>GAIRSDFSNEDIYDNIDPDTISFPPKIATTDLFLPLFFHFGSTRQFMDKLHEVISGDYEPSQAEKLVQDLCDETGIRKNFSTSILTCLSGDLMVFPRYFLNMFKDNVNPPPNVPGIWTHDDDESLKSNDQE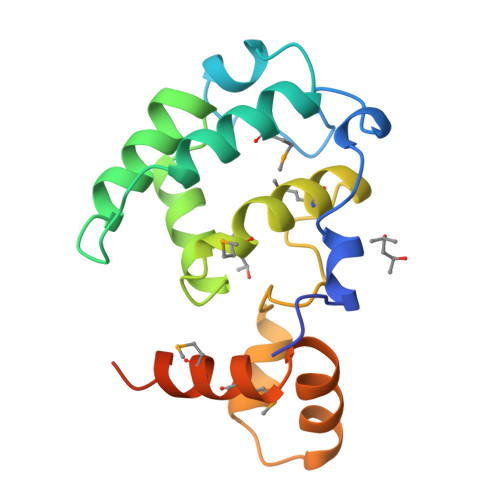QIRKLVKKHGTGRMEMRKRFFEKDLLVPRGSHHHHHH[2x]>[2x]MARKYFVAANWKCNGTLESIKSLTNSFNNLDFDPSKLDVVVFPVSVHYDHTRKLLQSKFSTGIQNVSKFGN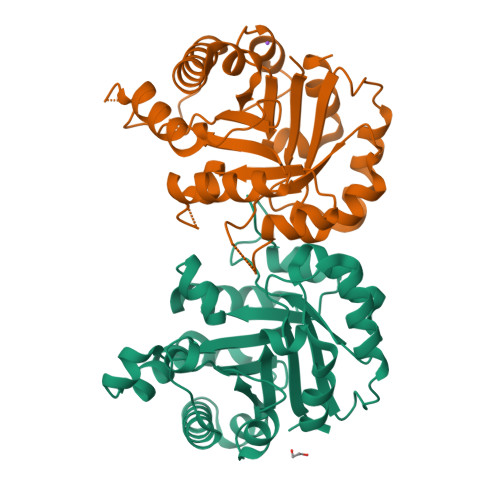GSYCGEVSAEIAKDLNIEYVIIGHFERRKYFHETDEDVREKLQASLKNNLKAVVCFGESLEQREQNKTIEVITKQVKAFVDLIDNFDNVILVYEPLWAIGTGKTATPEQAQLVHKEIRKIVKDTCGEKQANQIRILYGGSVNTENCSSLIQQEDIDGFLVGNASLKESFVDIIKSAM>MMNIIRKMDWDSMVHEYDLDGSRLLPWEGLNTPFGGAWCIVRPETKSFRHS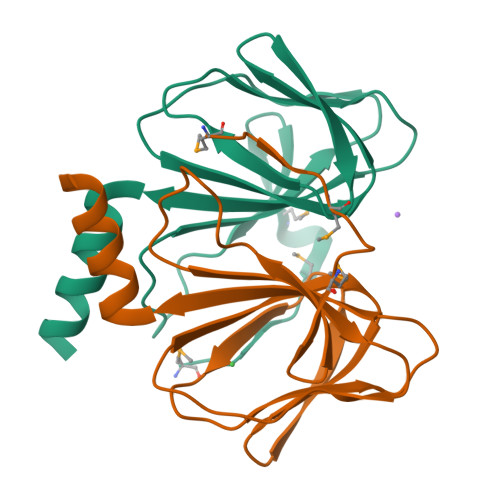HNEYELFIVIQGNAIIRINDEDFPVTKGDLIIIPLDSEHHVINNNQEDFHFYTIWWDKESTLNFLTRLEQDHHHHHH[2x]The oral bacterium Porphyromonas gingivalis, a “keystone” pathogen of periodontitis, produces a dual domain sialidase (PG0352). Biochemical analyses reveal that PG0352 can desialylate human serum and complement factors and thus protect bacteria from serum killing. Structural analyses show that PG0352 contains a N-terminal carbohydrate-binding module (CBM) and a C-terminal sialidase domain that exhibits a canonical six-bladed β-propeller sialidase fold with each blade composed of 3–4 antiparallel β-strands. Structural and functional analyses further demonstrate that the CBM binds to carbohydrates and serum glycoproteins.

To elucidate the catalytic mechanism of PG0352, we first determined its unliganded crystal structure using synchrotron radiation to 1.84Å in a monoclinic space group. Initial phases were obtained utilizing molecular replacement in conjunction with a model of the protein generated using AlphaFold2. The overall structure of PG0352 consists of two major domains encompassing 493 residues (31–523). We observed additional electron density within the active site pocket near the side chain of Tyr-488 that we subsequently modeled as a partially occupied citrate molecule derived from the crystallization cocktail (S4). One of the carboxyethyl groups of citrate interacts with Arg-194, Arg-398, and Arg-460, a triad of conserved arginine residues implicated in stabilizing the carboxylate group of sialic acid. Another carboxyethyl group interacts with the side chain of Arg-213, mimicking the interaction observed between this side chain and the O4 of sialic acid. This interaction perturbs the side chain of Asp-219, which exhibits alternate rotamer conformations in the unliganded structure. The third carboxyethyl group does not interact with the enzyme, given its orientation away from the active site pocket. Interestingly, the tartrate molecule observed in the sialidase active site of their structure binds in a virtually identical conformation to that observed for citrate bound in the unliganded PG0352 structure reported here, suggesting that these molecules may serve as useful stabilizing ligands to facilitate the crystallization of sialidase enzymes. The positions of the side chains of Tyr-488 and Glu-382 suggest that they serve as the nucleophile and the general base catalyst, respectively, as they occupy topologically equivalent positions in other structurally characterized bacterial sialidase enzymes.

> MRGSHHHHHHGSMQEVTMWGDSHGVAPNQVRRTLVKVALSESLPPGAKQIRIGFSLPKETEEKVTALYLLVSDSLAVRDLPDYKGRVSYDSFPISKEDRTTALSADSVAGRRFFYLAADIGPVASFSRSDTLTARVEEVAVDGRPLPLKELSPASRRLYRGYEALFVPGDGGSRNYRIPAILKTANGTLIAMADRRKYNQTDLPEDIDIVMRRSTDGGKSWSDPRIIVQGEGRNHGFGDVALVQTQAGKLLMIFVGGVGLWQSTPDRPQRTYISESRDEGLTWSPPRDITHFIFGKDCADPGRSRWLASFCASGQGLVLPSGRITFVAAIRESGQEYVLNNYVLYSDDEGDTWQLSDCAYRRGDEAKLSLMPDGRVLMSIRNQGRQESRQRFFALSSDDGLTWERAKQFEGIHDPGCNGAMLQVKRNGRDQVLHSLPLGPDGRRDGAVYLFDHVSGRWSAPVVVNSGSSAYSDMTLLADGTIGYFVEEGDEISLVFIRFVLDDLFDVRQ> SANEDMPVEKILEAELAVEPKTETYVEANMGLNPSSPNDPVTNICQAADKQLFTLVEWAKRIPHFSELPLDDQVILLRAG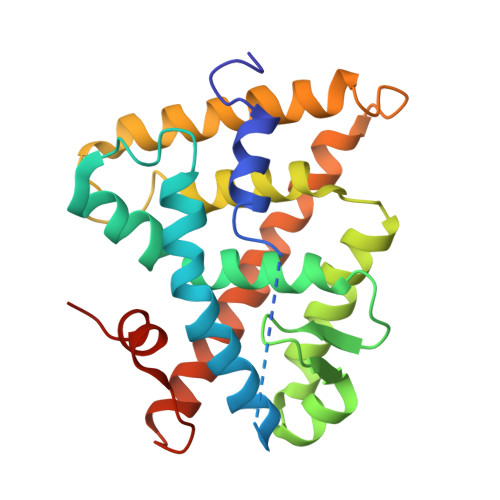WNELLIASFSHRSIAVKDGILLATGLHVHRNSAHSAGVGAIFDRVLTELVSKMRDMQMDKTELGCLRAIVLFNPDSKGLSNPAEVEALREKVYASLEAYCKHKYPEQPGRFAKLLLRLPALRSIGLKCLEHLFFFKLIGDTPIDTFLMEMLEAPHQAT>[7x]SKKQGDADVCGEVAY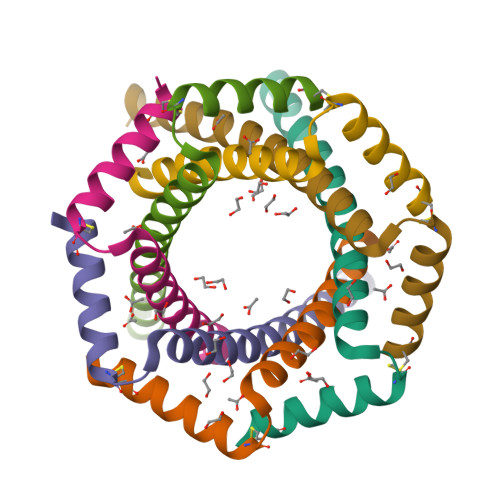IQSVVSDCHVPTEDVKTLLEIRKLFLEIQKLKVELQGLSKEFLEHILHGS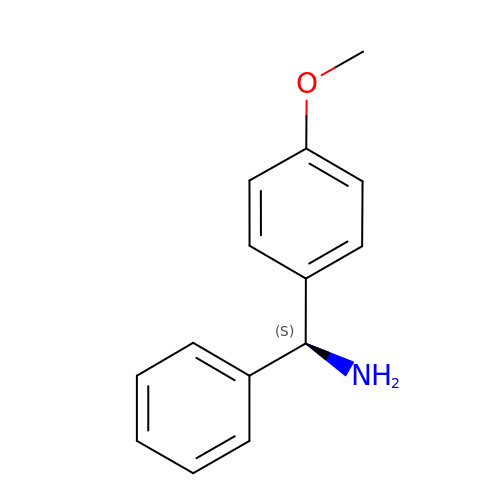(S)-1-(4-methoxyphenyl)-1-phenylmethanamine | C14 H15 N O | MXDBCXKVTJDKNP-UHFFFAOYSA-N>MAIAQLATEYVFSDFLLKEPTEPKFKGLRLELAVDKMVTCIAVGLPLLLISLAFAQEISIGTQISCFSPSSFSWRQAAFVDSYCWAAVQQKNSLQSESGNLPLWLHKFFPYILLLFAILLYLPPLFWRFAAAPHICSDLKFIMEELDKVYNRAIKAAKSARDLDMRDGACSVPGVTENLGQSLWEVSESHFKYPIVEQYLKTKKNSNNLIIKYISCRLLTLIIILLACIYLGYYFSL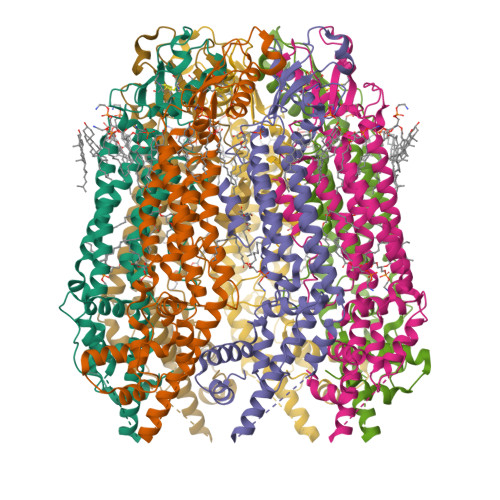SSLSDEFVCSIKSGILRADSTVPDQFQCKLIAVGIFQLLSVINLVVYVLLAPVVVYTLFVPFRQKTDVLKVYEILPTFDVLHFKSEGYNDLSLYNLFLEENISEVKSYKCLKVLENIKSSGQGIDPMLLLTNLGMI[7x]> MKKSKRKNAQAQEAQETEVLVQEEAEELPEFPEGEPDPDLEDPDLTLEDDLLDLPEEGEGLDLEEEEEDLPIPKISTSDPVRQYLHEIGQVPLLTLEEEVELARKVEEGMEAIKKLSEITGLDPDLIREVVRAKILGSARVRHIPGLKET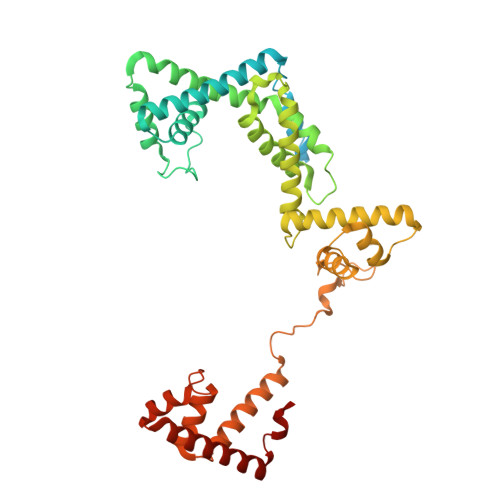LDPKTVEEIDQKLKSLPKEHKRYLHIAREGEAARQHLIEANLRLVVSIAKKYTGRGLSFLDLIQEGNQGLIRAVEKFEYKRRFKFSTYATWWIRQAINRAIADQARTIRIPVHMVETINKLSRTARQLQQELGREPTYEEIAEAMGPGWDAKRVEETLKIAQEPVSLETPIGDEKDSFYGDFIPDEHLPSPVDAATQSLLSEELEKALSKLSEREAMVLKLRKGLIDGREHTLEEVGAFFGVTRERIRQIENKALRKLKYHESRTRKLRDFLD> MRRTFISFSAASAAAAAPVTSTKMQTLHKLLTGEVSFKNKAPVKDCNIVHQFGENWATELSAYAKTLPAE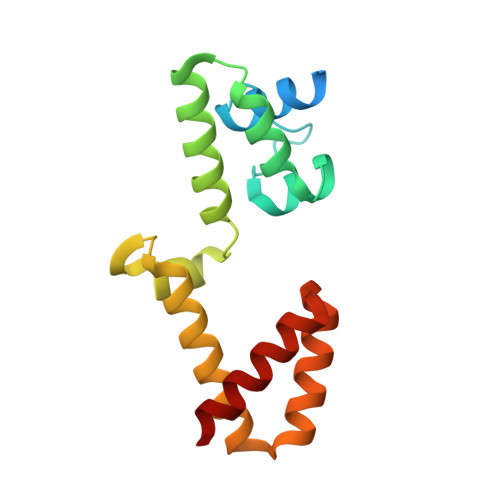QQKIIVRQIARVKLTRYTVAELAAYCGDGPALLDETARAANIEQGVAFVKAKGVEAFEKYVAEESTNANWKPEEAKKFIEDVKAKAK>HSAGVTALVPSLLNNGTEQIAVQPVPQIPFPVFNDPFLHELEKLRRESENSKKTFEEKKSILKAELERKMAEVQAEFRRKFHEVEAEHNTR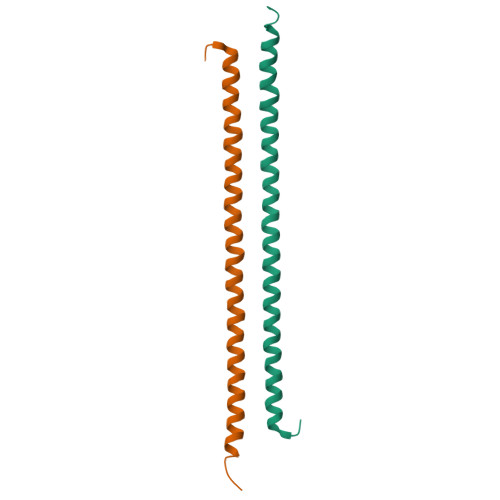TTKIEKDKNLVIMNKLLANAFLSK[4x]3-(3-methylindol-1-yl)propanoic acid | C12 H13 N O2 | 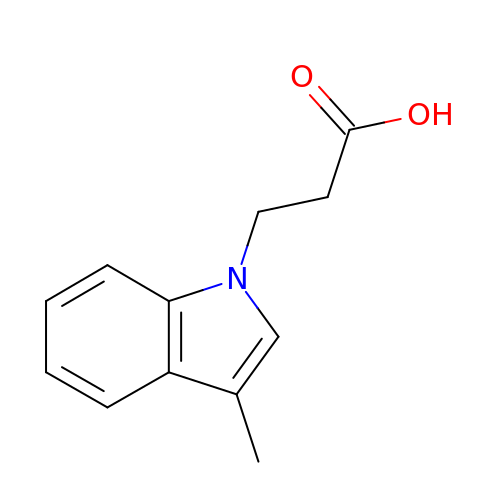YJMBLVFDTDJZFE-UHFFFAOYSA-N>[2x]MRHPLVMGNWKLNGSRHMVHELVSNLRKELAGVAGCAVAIAPPEMYIDMAKREAEGSHIMLGAQNVDLNLSGAFTGETSAAMLKDIGA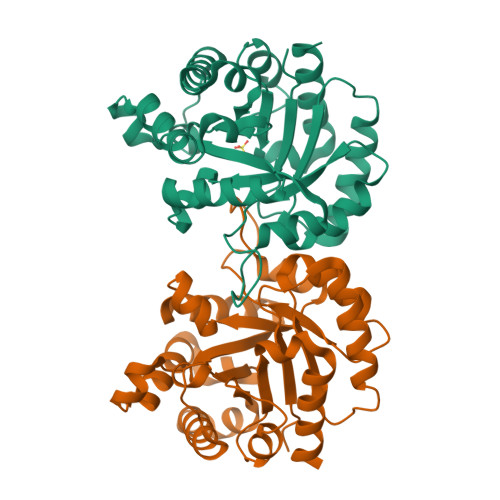QYIIIGHSERRTYHKESDELIAKKFAVLKEQGLTPVLCIGETEAENEAGKTEEVCARQIDAVLKTQGAAAFEGAVIAYEPVWAIGTGKSATPAQAQAVHKFIRDHIAKVDANIAEQVIIQYGGSVNASNAAELFAQPDIDGALVGGASLKADAFAVIVKAAEAAKQA> MPLTEHLRELRYRLIISIIAFLIGSGIAFYFAKYVFEILKEPILKSYPEVELITLSPTEPLFILIKISLAVGFIIASPVILYQFWRFIEPALYSHEKRAFIPLLLGSILLFMLGALFAYFIVLPLALKFLL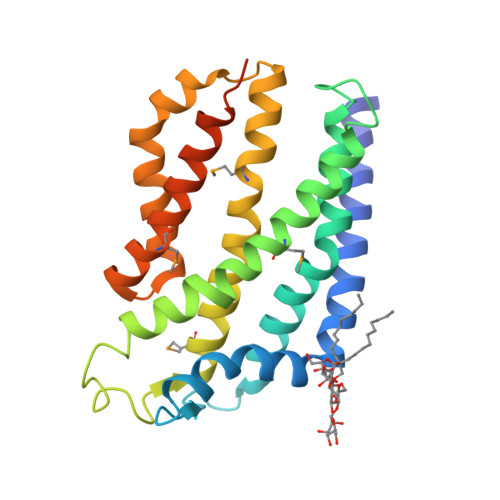GLGFTQLLATPYLSVDMYISFVLKLVVAFGIAFEMPIVLYVLQKAGVITPEQLASFRKYFIVIAFVIGAIIAPDVSTQVLMAIPLLLLYEISIFLGKLATRKKKEIQKAPGSENLYFQ> MPQLPEVETIRRTLLPLIVGKTIEDVRIFWPNIIRHPRDSEAFAARMIGQTVRGLERRGKFLKFLLDRDALISHLRMEGRYAVASALEPLEPHTHV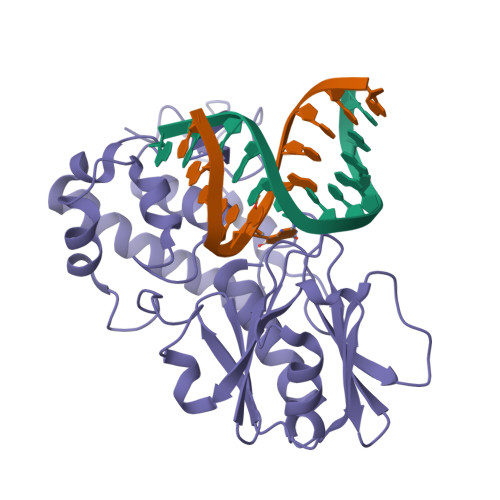VFCFTDGSELRYRDVRKFGTMHVYAKEEADRRPPLAELGPEPLSPAFSPAVLAERAVKTKRSVKALLLDQTVVAGFGNIYVDESLFRAGILPGRPAASLSSKEIERLHEEMVATIGEAVMKGGSTVRTYVNTQGEAGTFQHHLYVYGRQGNPCKRCGTPIEKTVVAGRGTHYCPRCQR> AEDVYQNFEELKNNEDPSDYGVVTKETGSPVLVLAIHGGGIEGGTSEVARELSKEYSMYLFEGLKSAGNSVLHITSTHFDEPRALKMTGNHEYVISLHGYAEEDQQIEVGGTDRVRAADLVEKLQHAGFPAVLLNMDHPHAGVSPNNIANKSKTGLSIQIEMSTGFRKSLFGIFSLKSRAVTQNERFYEFTEVMFRFLKNSYLE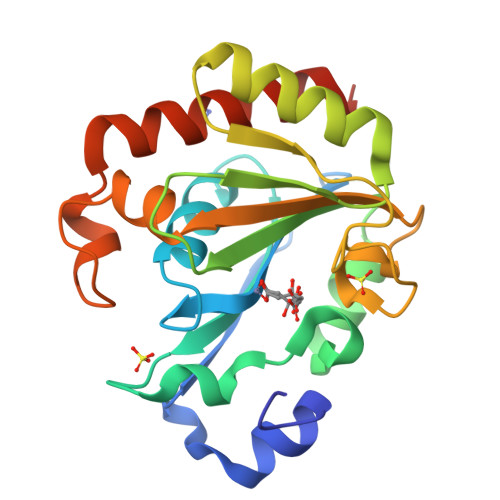HHHHHH> SQPACTARRRTRVLILGVNGFIGNHLTERLLREDHYEVYGLDIGSDAISRFLNHPHFHFVEGDISIHSEWIEYHVKKCDVVLPLVAIATPIEYTRNPLRVFELDFEENLRIIRYCVKYRKRIIFPSTSEVYGMCSDKYFDEDHSNLIVGPVNKPRWIYSVSKQLLDRVIWAYGEKEGLQFTLFRPFAWMGPRLDNLNAARIGSSRAITQLILNLVEGSPIKLIDGGKQKRCFTDIRDGIEALYRIIENAGNRCDGEIINIGNPENEASIEELGEMLLASFEKHPLRHHFPPFA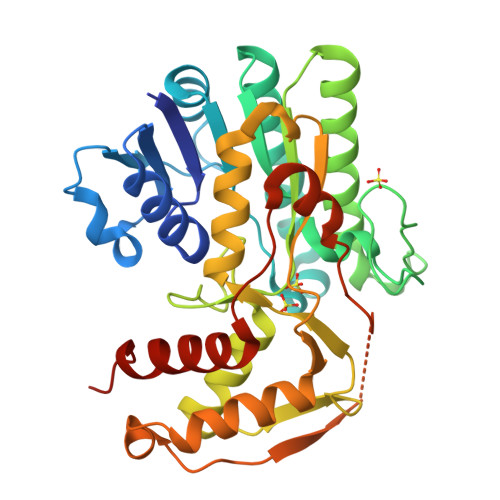GFRVVESSSYYGKGYQDVEHRKPSIRNAHRCLDWEPKIDMQETIDETLDFFLRTVDLTDKPS>GSFTMASMTGGQQMGRGSMNGDVQSVIRGYLERAQVAKTMSDAGRWNEAGDLLRQLMTDVKSCKISASNRDEHDARNTFLRALEANLKLVQQNVRDEDDLHEAMTRQSGSPEPPADPDVWSKPSPPLPSSSKFGATKKGVGAAGPRPREISKSTSSMSTNPADVKPANPTQGILPQNSAGDSFDASAYDAYIVQAVRGTMATNTENTM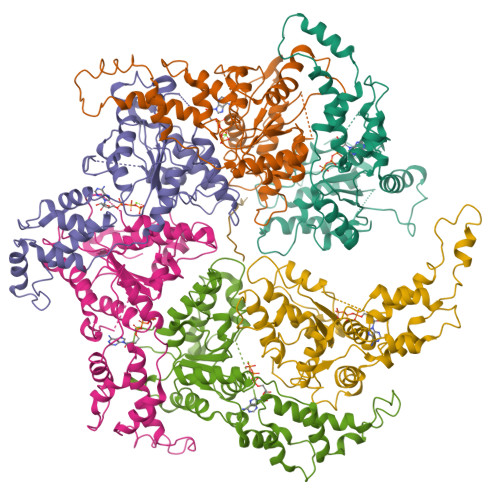SLDDIIGMHDVKQVLHEAVTLPLLVPEFFQGLRSPWKAMVLAGPPGTGKTLIARAIASESSSTFFTVSSTDLSSKWRGDSEKIVRLLFELARFYAPSIIFIDQIDTLGGQRGNSGEHEASRRVKSEFLVQMDGSQNKFDSRRVFVLAATNIPWELDEALRRRFEKRIFIPLPDIDARKKLIEKSMEGTPKSDEINYDDLAARTEGFSGADVVSLCRTAAINVLRRYDTKSLRGGELTAAMESLKAELVRNIDFEAALQAVSPSAGPDTMLKCKEWCDSFGAM[6x];> EEEEEEEEEEEEEE>[2x]KTEMKDDFAKLEEQFDAKLGIFALDTGTNRTVAYRPDERFAFASTIKALTVGVLLQQKSIEDLNQRITYTRDDLVNYNPITEKHVDTGMTLKELADASLRYSDNAAQNLILKQIGGPESLKKELRKIGDEVTNPERFEPELNEVNPGETQDTSTARALVTSLRAFALEDKLPSEKRELLIDWMKRNTTGDALIRAGVPDGWEVADK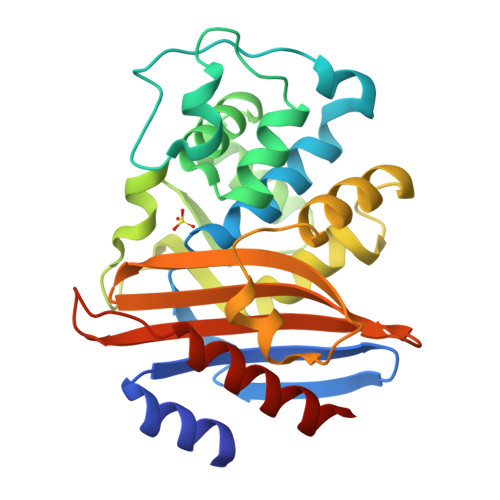TGAASYGTRNDIAIIWPPKGDPVVLAVLSSRDKKDAKYDDKLIAEATKVVMKALNMNGK> MSLLERGLSKLTLNAWKDREGKIPAGSMSAMYNPETIQLDYQTRFDTEDTINTASQSNRYVISEPVGLNLTLLFDSQMPGNTTPIETQLAMLKSLCAVDAATGSPYFLRITWGKMRWENKGWFAGRARDLSVTYTLFDRDATPLRATVQLSLVADESFVIQQSLKTQSAPDRALVSVPDLASLPLLALSAGGVLASSVDYLS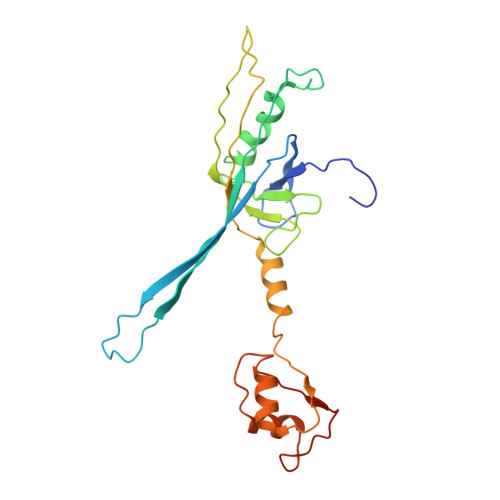LAWDNDLDNLDDFQTGDFLRATKGEEV>MPPKARAPLPPGDAARGEKLFKGRAAQCHTANQGGANGVGPNLYGLVGRHSGTIEGYAYSKANAESGVVWTPDVLDVYLENPKKFMPGTKMSFAGM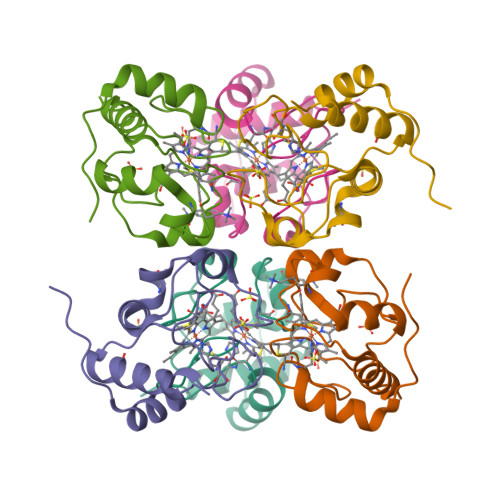KKPQERADVIAYLETLKG[3x]7-O-phosphono-D-glycero-beta-D-manno-heptopyranose 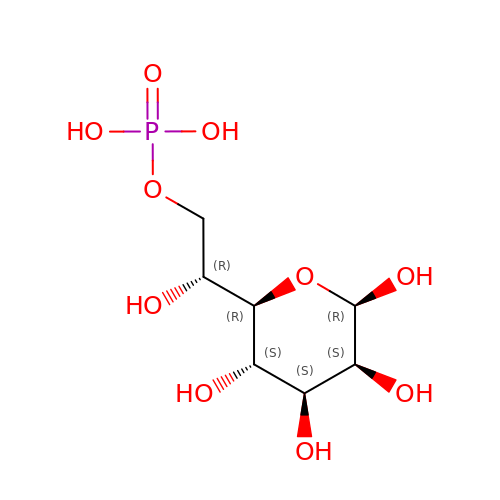| C7 H15 O10 P | SDADNVAZGVDAIM-ZUHYCWGWSA-N Here, we demonstrate that Rv3722c is the primary aspartate aminotransferase (AspAT) in Mtb, non-redundantly catalyzes the specific biosynthesis of Asp in vitro, and is essential for axenic growth and survival of Mtb in macrophages and in mice. The overall fold of Rv3722c is similar to that of other members of the recently described type Ic subgroup of PLP-binding proteins. Each monomer consists of a core domain (Pro52-Gly302) that folds into a nearly perfect α/β motif comprised a central eight-stranded (predominantly antiparallel) β-sheet surrounded by eight α-helices. Rv3722c also contains an N-terminal auxiliary domain (Ser2-Leu53 and Asp303-Ser430) that stacks and forms an elongated segment on top of the core domain, and consists of five α-helices and an antiparallel β-sheet.

In the asymmetric unit of Rv3722c pre-incubated with Kyn, we observed that the chains were bound to either the external aldimine intermediate PLP-kynurenine (PLP-Kyn), or the final keto acid product kynurenic acid (Kyna). In the unbound form of Rv3722c, the positively charged guanidinium side chain of Arg36 points outward and lies above the entrance of the active site pocket. Upon binding Kyn, however, we observed that the side chain of this residue is positioned more inward (by ~12 Å measured from the Cζ atom) and interacts with Kyn. Upon moving inward, Arg36 forms a bidentate salt bridge with Asp140. This ligand-induced conformational change is reminiscent of the so called “arginine switch” observed in type Ia AspATs, although here the Arg residue moves toward the substrate rather than away. In our structure, we observed a sharp peak of a water molecule in close proximity to both the active site Lys257 and the PLP-KYN intermediate. We speculate that this is the same water molecule responsible for the generation of the keto acid Kyna, from the PLP-KYN intermediate. When compared with Kyn, the carboxylate moiety of Kyna is rotated by ~180° and faces the entrance of the solvent-exposed binding pocket. Interestingly, in all the Kyna-bound chains, Arg36 adopts its original “outward” conformation, most likely facilitating the release of the product. Our data thus show that the aliphatic backbone of Kyn mimics the dicarboxylic amino acid Asp, and provide a possible explanation why Rv3722c—and potentially other AspATs—display side activity towards the structurally disparate Kyn.

>[8x]VSFDSLSPQELAALHARHQQDYAALQGMKLALDLTRGKPSAEQLDLSNQLLSLPGDDYRDPEGTDTRNYGGQHGLPGLRAIFAELLGIAVPNLIAGNNSSLELMHDIVAFSMLYGGVDSPRPWIQEQDGIKFLCPVPGYDRHFAITETMGIEMIPIPMLQDGPDVDLIEELVAVDPAIKGMWTVPVFGNPSGVTYSWETVRRLVQMRTAAPDFRLFWDNAYAVHTLTLDFPRQVDVLGLAAKAGNPNRPYVFASTSKITFAGGGVSFFGGSLGNIAWYLQYAGKKSIGPDKVNQLRHLRFFGDADGVRLHMLRHQQILAPKFALVAEVLDQRLSESKIASWTEPKGGYFISLDVLPGTARRTVALAKDVGIAVTEAGASFPYRKDPDDKNIRIAPSFPSVPDLRNAVDGLATCALLAATETLLNQGLASSAPNVR>[2x]MKYNTGAGTVPEQLNVHLVPHSHDDVGWLKTVDQYYVGSENYIQEACVENVLDSVVMSLQRDPNRKFVFGEMAFFHRWWLEQTPETKELVRKLVKAGQLEFVNGGWCMHDEATTHYIDMIDHTTLGHRFIQEQFNKIPRAGWQIDPFGHSAVQGYLLGAELGFDSVHFARIDYQDREKRKAEKSLEVVWRGSKTFGSSAQIFANAFPGHYGPPNGFNFEVRNNFVPLQDDPRLFDTNVEERVQNFIDAALTQAKITRTNHIMWTMGDDFQYQYAESWFKQMDKLIHHVNKDGRVNALYSTPSIYTEAKNAANQTWPLKIDDYFPYADGRN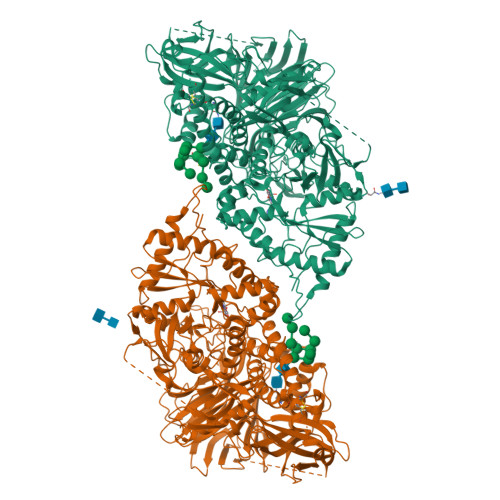AYWTGFYTSRSALKDYVRMLSGYYLATRQLGFFAGKKSTKYHAFDLADALGIAQHHDAVSGTAKQHTTNDYAKRLAIGASKAEAVVSSSLACLTSKQSADQCSAPASAFSQCHLFNISYCPPTESSIPDDKSLVVVVYNPLGWSRNEIVRIPVNDANLVVKDSSGNKLEVQYVEMDDVTANLRSFYVKAYEGEVPKDADVYWSLFKASVPPLGWSTYFISEATGKGTRNALTLSQKGETLNIGPGDLKMSFSSLTGQLKRMYNSKTGVDIPIQQNYLWYESSEGDFSDYQASGAYIFRPNGQPPPHTVSRSSVTRVTRGPLVDEVHQKFNSWISQVTRLYKDKDHAEIEFTIGPIPTDDGVGKEVITRMTSTMATNKEFYTDSNGRDFLKRVRDYREDWPLEVTQPVAGNYYPLNLGIYTKDEKSEFSVLVDRATGGASIKDGEVELMLHRRTIRDDGRGVGEPLDEQVCMNKEYTCEGLTVRGNYYLSIHKPAAGSRWRRTTGQEIYSPMLLAFTQENMENWKSSHSTKGIFMDPNYSLPPSVALITLEELDDGLVLLRLAHLYEPSEDAEYSTLTKVELKKLFATQKIEELREVSLSANQEKSEMKKMKWSVEGDNEQEPQAVRGGPVSNADFVVELGPMEIRTFLLQF> XYGHSHIRFGYSYH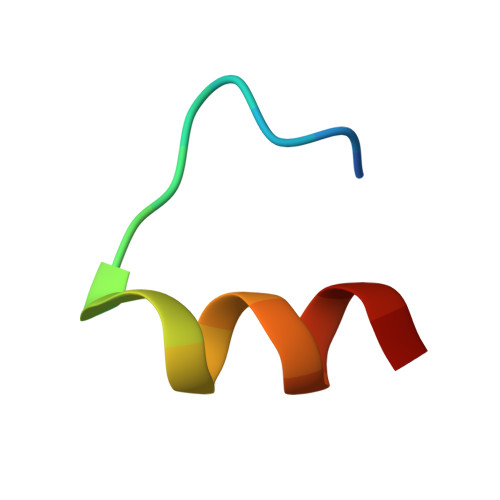VSYCGX>[2x]MGSSHHHHHHSSENLYFQGGGHMDYKILNFDAKNDNRGSLIALENLKEIPFEIKRIYYIYDTKP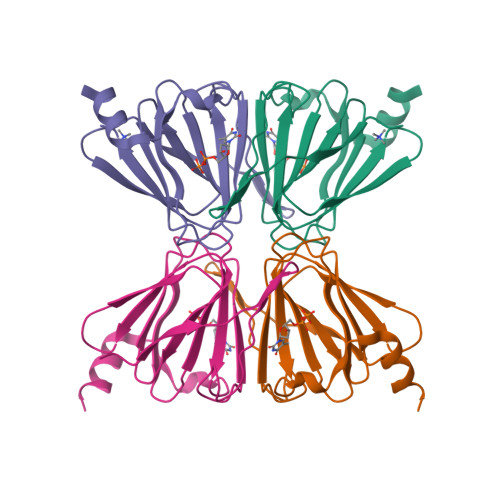DFPRGAHAHKELEQVLIMMDGSCEIVLNDGRNDKSIILNRPNIGLFIGKNMWREMRNFSYGAKLLVLASDFYNENEYIRDYDEFLRMVNDT5-{2-[1-(1-METHYL-PROPYL)-7A-METHYL-OCTAHYDRO-INDEN-4-YLIDENE]-ETHYLIDENE}-2-METHYLENE-CYCLOHEXANE-1,3-DIOL | C23 H36 O2 | 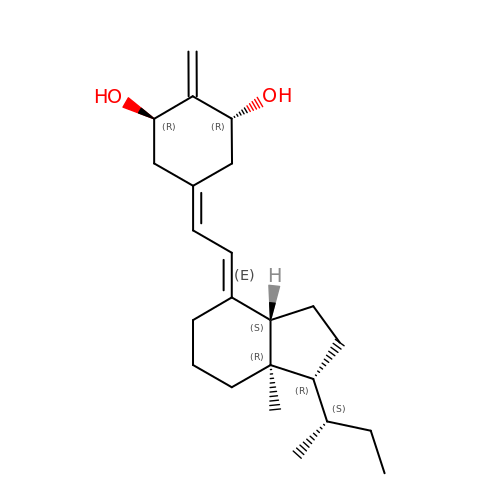QSLUXQQUPXBIHH-YHSKWIAJSA-N> WTPFSWVEKYAYAFSGPYNKAEVALTFDDGPDLEFTPKILDKLKQHNVKATFFLLGENAEK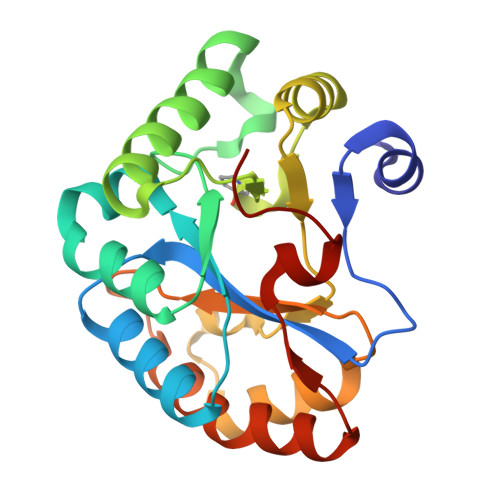FPNIVKRIANEGHVIGNHTYSHPNLAKVNEDEYRNQIIKTEEILNRLAGYAPKFIRPXYGEILENQLKWATEQNFMIVQWSVDTVDWKGVSADTITNNVLGNSFPGSVILQHSTPGGHLQGSVDALDKIIPQLKTKGARFVTLPSMFQTSKER>[2x]KAFPVLGIDYTHVRTPFEISLWILLACLMKIGFHVIPTISSIVPESCLLIVVGLLVGGLIKGVGETPPFLQSDVFFLFLLPPIILDAGYFLPLRQFTENLGTILIFAVVGTLWNAFFLGGLMYAVCLVGGEQIN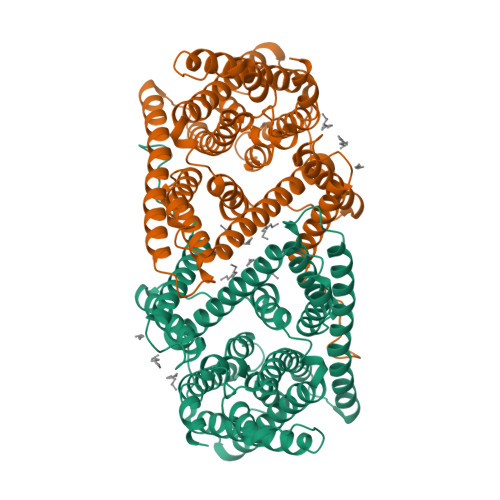NIGLLDNLLFGSIISAVDPVAVLAVFEEIHINELLHILVFGESLLNDAVTVVLYHLFEEFANYEHVGIVDIFLGFLSFFVVALGGVLVGVVYGVIAAFTSRFTSHIRVIEPLFVFLYSYMAYLSAELFHLSGIMALIASGVVMRPYVEANISHKSHTTIKYFLKMWSSVSETLIFIFLGVSTVAGSHHWNWTFVISTLLFCLIARVLGVLGLTWFINKFRIVKLTPKDQFIIAYGGLRGAIAFSLGYLLDKKHFPMCDLFLTAIITVIFFTVFVQGMTIRPLVDLL methyl {3-[2-(acetylamino)ethyl]-1H-indol-5-yl}carbamate 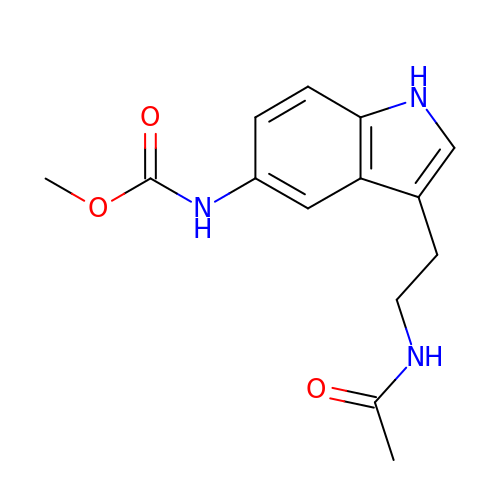| C14 H17 N3 O3 | MPZVHKLZCUEJFO-UHFFFAOYSA-N>[2x]SKTRQTFSWV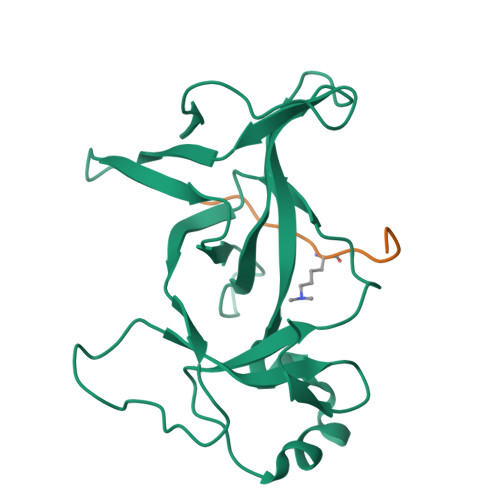GRPLPNRKQFQQMYREICMKINDGSEIHIKVGQFVLIQGEDNKKPYVAKLIELFQNGAEVPPKKCARVQWFVRFLEIPVSKRHLLGRSPPAQEIFWYDCSDWDNKINVETIIGPVQVVALAPEEVIPVDQKSEETLFVKLSWNKKDFAPLPPE;>GAKRHRKVLRDN[2x]> MYGSKTFIKYVSGIPDYFKQSFPEGFTWERTTTYEDGGFLTAHQDTSLDGDCLVYKVKILGNNFPADGPVMQNKAGGWEPSCEILYEVDGVLCGQSLMALKCPGGRHLNCRLHTTYRSKKPASALKMPEFHFEDHRIEVKEVQKGK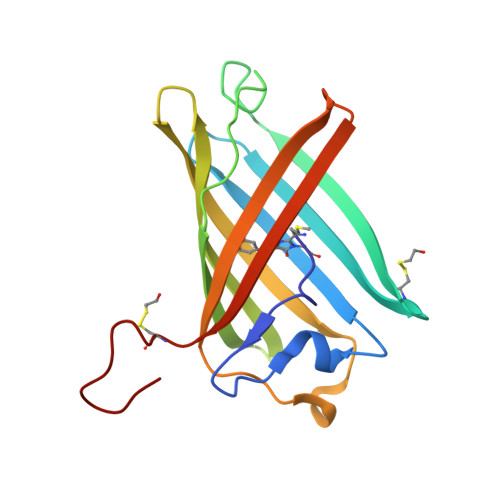HYEQYEAAVARYCDAAPSKLGHH> MDDMQVYIANLGKYNEGELVGAWFTFPIDFEEVKEKIGLNDEYEEYAIHDYELPFTVDEY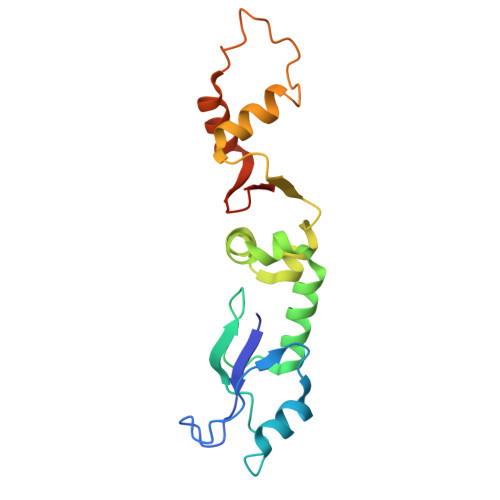TSIGELNRLWEMVSELPEELQSELSALLTHFSSIEELSEHQEDIIIHSDCDDMYDVARYYIEETGALGEVPASLQNYIDYQAYGRDLDLSGTFISTNHGIFEIVY> MATLRVHPEAQAKVDVFREDLCSKTENLLGSYFPKKISELDAFL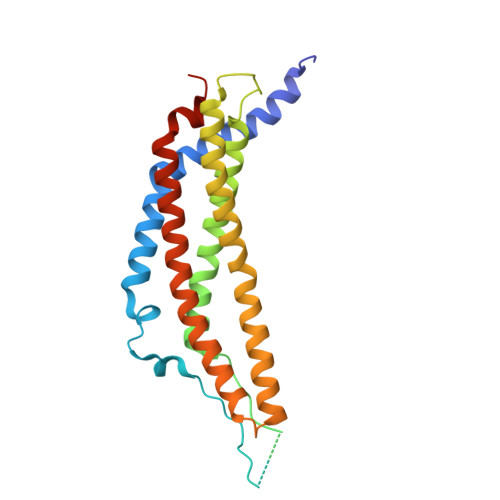KEPALNEANLSNLKAPLDIPVPDPVKEKEKEERKKQQEKEEKEEKKKGDEDDKGPPCGPVNCNEKIVVLLQRLKPEIKDVTEQLNLVTTWLQLQIPRIEDGNNFGVAVQEKVFELMTNLHTKLEGFHTQISKYFSERGDAVAKAAKQPHVGDYRQLVHELDEAEYQEIRLMVMEIRNAYAVLYDIILKNFEKLKKPRGETKGMIY> LGGDRDFWLQVGIDPIQIMTGTATFYTLRCYLDDRPIFLGRNGRISVFGSERALARYLADEHDHDLSDLSTYDDIRTAATDGSLAVAVTDDNVYVLSGLVDDFADGPDAVDREQLDLAVELLRDIGDYSEDSAVDKALETTRPLGQLVAYVLDPHSVGKPTAPYAAAVREWEKLERFVESRLRRE

Here, we demonstrated that SatS, which we revealed is required for M. tuberculosis growth in macrophages, functions in the export of SapM and an additional subset of the proteins exported by the SecA2 pathway. We further identified properties of SatS that indicate a function as a protein export chaperone that protects its substrates from inappropriate interactions in the cytoplasm and additionally assists in their export. SatS is a highly acidic (pI 3.83), cytoplasmic protein with a role promoting export of a subset of the proteins exported by the SecA2 pathway. Finally, we determined the structure of the C-domain of SatS (SatSC), which reveals a new fold lacking similarities to any solved chaperone structures, yet contains surface hydrophobic grooves resembling those of the SecB chaperone.

To gain further insight into SatS function, we collected diffraction quality crystals and determined the crystal structure of SatS to 2.3 Å. Upon inspection, the electron density map only corresponded to the last 185 amino acids (L237-E420) C-domain of the SatS sequence (SatSC). The molecular weight of the SatSC crystal was ~25 kDa as determined by SDS-PAGE, indicating that the protein underwent in situ proteolysis in the crystallization buffer. Although we set out to solve the structure of SatS in its entirety, we were only able to obtain structural information for the C-terminal half of the protein (SatSC), which arose during crystallization. Further investigation revealed striking similarity between the experimentally derived SatSC secondary structure and the predicted secondary structure of the first ~180 amino acids of the N-domain of SatS (SatSN). The SatSC and SatSN domains are also similar in size with 41% sequence similarity at the amino acid level. This raised the possibility that SatS is comprised of two similar domains with an intervening ~60 amino acids that is predicted to be a flexible, disordered linker. However, the primary sequence and secondary structure similarity between the N-terminal and C-terminal halves of SatS raise the possibility of SatS being comprised of tandem SatSC-like domains. SatSC displays α/β secondary structure comprised of a mostly parallel, four stranded β-sheet core, flanked by seven α-helices. Investigation of the SatSC structure revealed a large network of negatively charged amino acids surrounding two surface exposed hydrophobic grooves, which are similar in arrangement, shape and size to the hydrophobic client binding sites of a SecB monomer.>MHPKIFALLAKFPRVELIPWETPIQYLPNISREIGADVYIKRDDLTGLGIGGNKIRKLEYLLGDALSKGADVVITVGAVHSNHAFVTGLAAKKLGLDAILVLRGKEELKGNYLLDKIMGIETRVYDAKDSFELMKYAEEIAEELKREGRKPYVIPPGGASPIGTLGYVRAVGEIATQSEVKFDSIVVAAGSGGTLAGLSLGLSILNEDIRPVGIAVGRFGEVMTSKLDNLIKEAAELLGVKVEVRPELYDYSFGEYGKITGEVAQIIRKVGTREGIILDPVYTGKAFY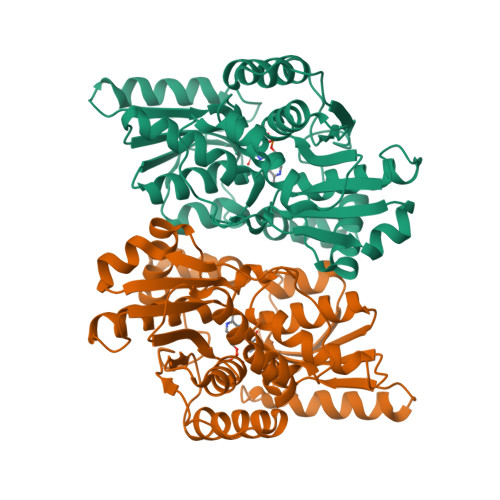GLVDLARKGELGEKILFIHTGGISGTFHYGDKLLSLL[24x]>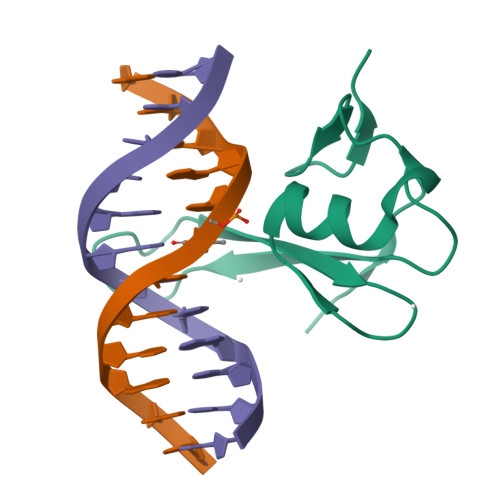GATESGKRMDCPALPPGWKKEEVIRKSGLSAGKSDVYYFSPSGKKFRSKPQLARYLGNTVDLSSFDFRTGKMMPSKLQK[6x]> SAGTSVTLQLDDGSGRTYQLREGSNIIGRGQDAQFRLPDTGVSRRHLEIRWDGQVALLADLNSTNGTTVNNAPVQEWQLADG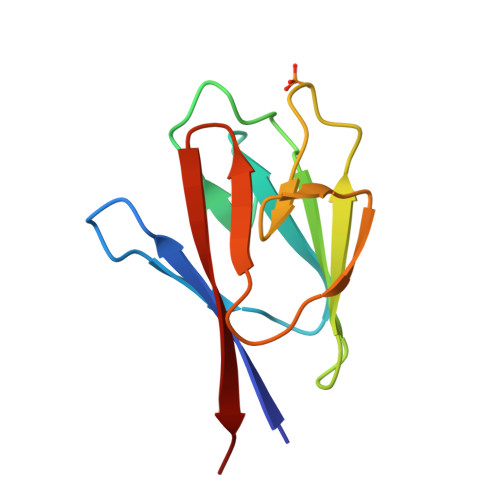DVIRLGHSEIIVRMHPLT> QQFFFENDALGQSSTDFATNFLNLWDNNREQLLNLYSPQSQFSVSVDSTIPPSTVTDSDQTPAFGYYMSSSRNISKVSSEKSIQQRLSIGQESINSIFKTLPKTKHHLQEQPNEYSMETISYPQINGFVITLHGFFEETGKPELESNKKTGKNNYQKNRRYNHGYNSTSNNKLSKKSFDRTWVIVPMNNSVIIASDLLTVRAYSTGAWKTAS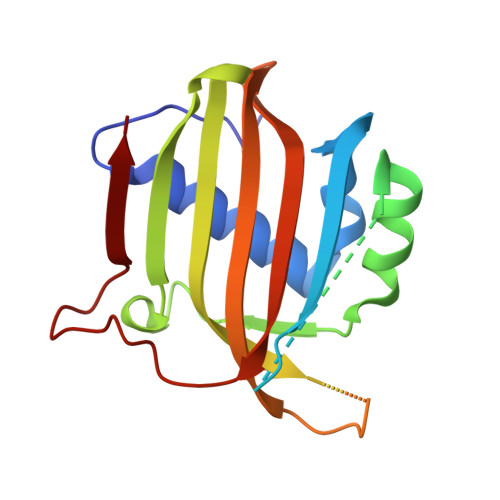IAIAQAAGS>MEKTRVNGTDRPPISSWSVDDVSNFIRELPGCQDYVDDFIQQEIDGQALLLLKEKHLVNAMGMKLGPARKIVAKVESIKEVRDHHHHHH[2x];>[2x]MEKTRANSHLRSQPIDWTIEEVIQYIESNDNSLAVHGDLFRKHEIDGKALLRLNSERMMKYMGLKLGPALKICNLVN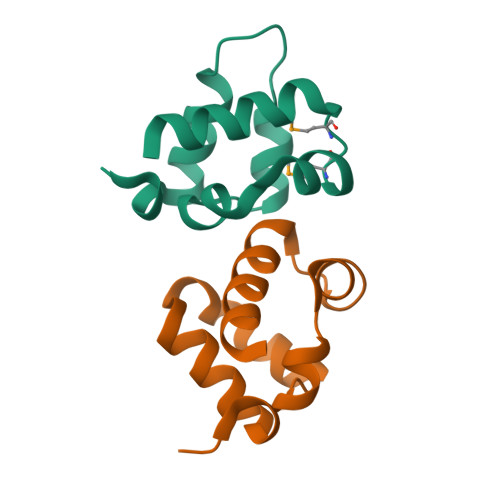KVNGRDHHHHHH>[2x]MPSVKIGIIGAGSAVFSLRLVSDLCKTPGLSGSTVTLMDIDEERLDAILTIAKKYVEEVGADLKFEKTMNLDDVIID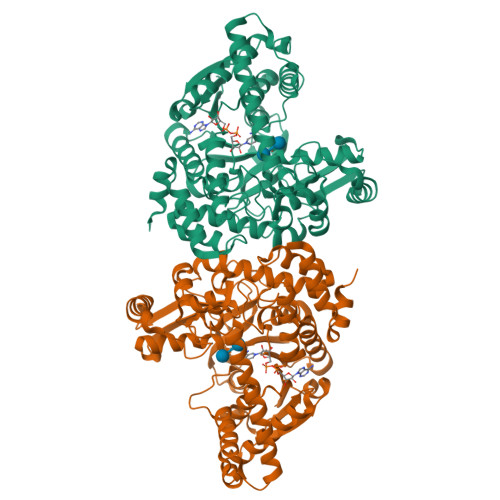ADFVINTAMVGGHTYLEKVRQIGEKYGYYRGIDAQEFNMVSDYYTFSNYNQLKYFVDIARKIEKLSPKAWYLQAANPIFEGTTLVTRTVPIKAVGFCHGHYGVMEIVEKLGLEEEKVDWQVAGVNHGIWLNRFRYNGGNAYPLLDKWIEEKSKDWKPENPFNDQLSPAAIDMYRFYGVMPIGDTVRNSSWRYHRDLETKKKWYGEPWGGADSEIGWKWYQDTLGKVTEITKKVAKFIKENPSVRLSDLGSVLGKDLSEKQFVLEVEKILDPERKSGEQHIPFIDALLNDNKARFVVNIPNKGIIHGIDDDVVVEVPALVDKNGIHPEKIEPPLPDRVVKYYLRPRIMRMEMALEAFLTGDIRIIKELLYRDPRTKSDEQVEKVIEEILALPENEEMRKHYLKR> GSHMKNSVSVDLPGSMKVLVSKSSNADGKYDLIATVDALELSGTSDKNNGSGVLEGVKADASKVKLTISDDLGQTTLEVFKSDGSTLVSKKVTSNGSSTEERADGTRLEYTGIKSDGSGKAKEVLKGYVLEGTLTAEKTTLVVKEGTVTLSKNISKSGEVSVELNDTDSSAATKKTAAWNSG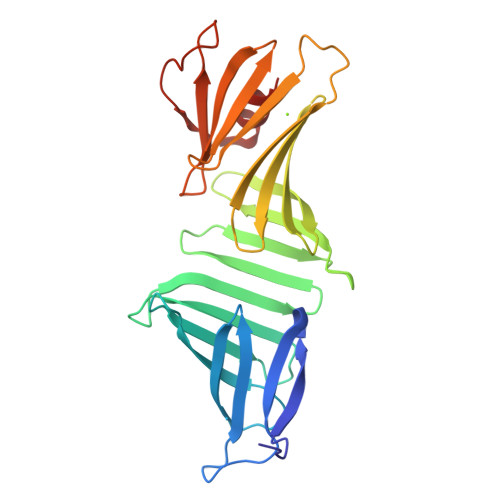TSTLTITVNSKKTKDLVFTSSNTITVQQYDSNGTSLEGSAVEITKLDEIKNALK>EAEAEFQTSCEQYAVFSGGNGYSVSNNLWGQSAGSGFGCITVNSLNSAASWHADWQWSGGQNNVKSYPNVQIAIPQKRIVNSIGSMPTTASWSYTGSNLRADVAYDLFTASNPNHVTYSGDYELMIWLARYGDIGPIGSAQGTVTINGQSWTLYYGFNGAMQVYSFVAPSTVTNWSGDVKNFFNYLRDNKGYPASSQYVLSYQFGTEPFTGSGTLNVNSW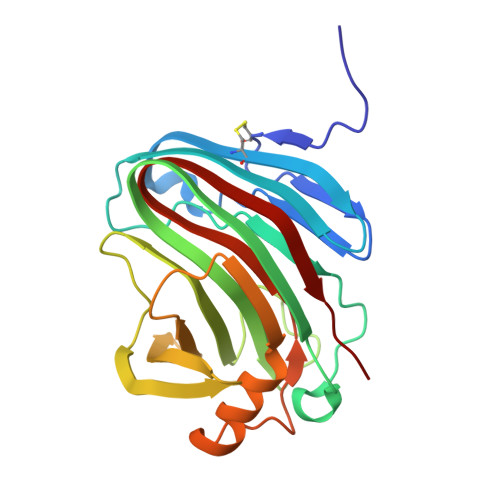TASINV[2x]>ARSTNTFNYATYHTLDEIYDFMDLLVAEHPQLVSKLQIGRSYEGRPIYVLKFSTGGSNRPAIWIDLGIHSREWITQATGVWFAKKFTEDYGQDPSFTAILDSMDIFLEIVTNPDGFAFTHSQNRLWRKTRSVTSSSLCVGVDANRNWDAGFGKAGASSSPCSETYHGKYANSEVEV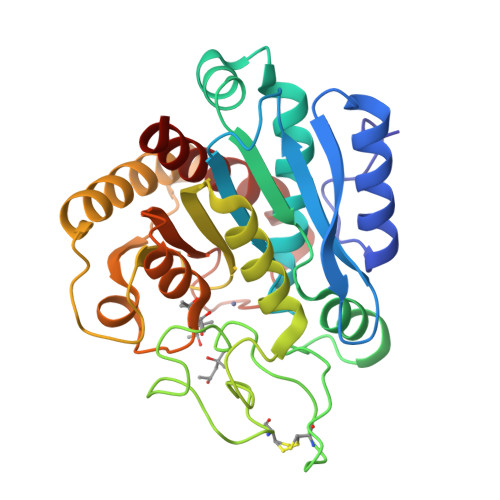KSIVDFVKDHGNFKAFLSIHSYSQLLLYPYGYTTQSIPDKTELNQVAKSAVAALKSLYGTSYKYGSIITTIYQASGGSIDWSYNQGIKYSFTFELRDTGRYGFLLPASQIIPTAQETWLGVLTIMEHTVNNLY[2x]>[2x]MALSAEGSSGGSRGGSPKAEAASVPSWPQILGRLTDNRDLARGQAAWAMDQIMTGNARPAQIAAFAVAMTMKAPTADEVGELAGVMLSHAHPLPADTVPD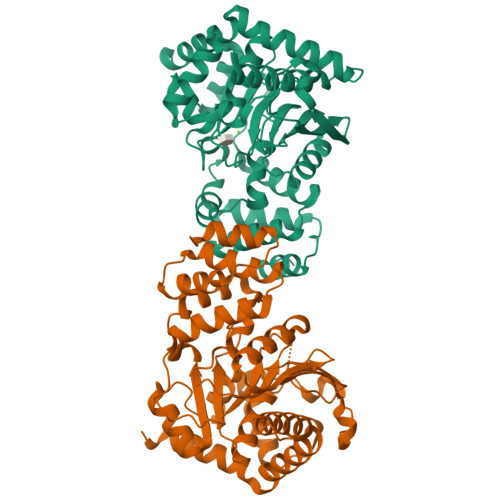DAVDVVGTGGDGVNTVNLSTMAAIVVAAAGVPVVKHGNRAASSLSGGADTLEALGVRIDLGPDLVARSLAEVGIGFCFAPRFHPSYRHAAAVLREIGVPTVFNLLGPLTNPARPRAGLIGCAFADLAEVMAGVFAARRSSVLVVHGDDGLDELTTTTTSTIWRVAAGSVDKLTFDPAGFGFARAQLDQLAGGDAQANAAAVRAVLGGARGPVRDAVVLNAAGAIVAHAGLSSRAEWLPAWEEGLRRASAAIDTGAAEQLLARWVRFGRQILEHHHHHH> MSFRTHLESVVNQVEGALACSVMGF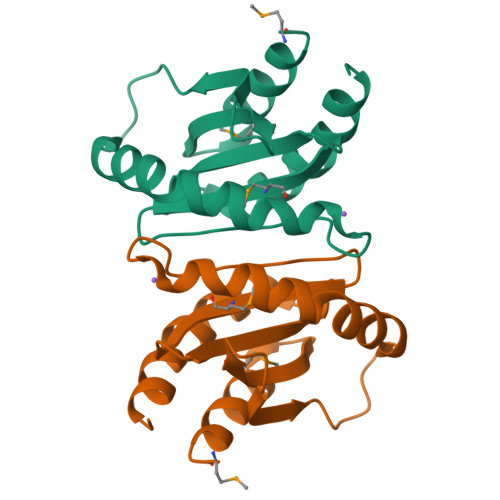DGISVDTFQKDESAELDLNGAWVEYANLLTQLRNAAETLKTGTVSEVSVNSEKVLTVMRLVSPDYFLVLALHADGNFGKGRYVLRVTAPKVRAEL2-{[(2-{[(E)-2-(dimethylamino)ethenyl](ethyl)amino}-2-oxoethyl)amino]methyl}pyridine-4-carboxylic acid | C15 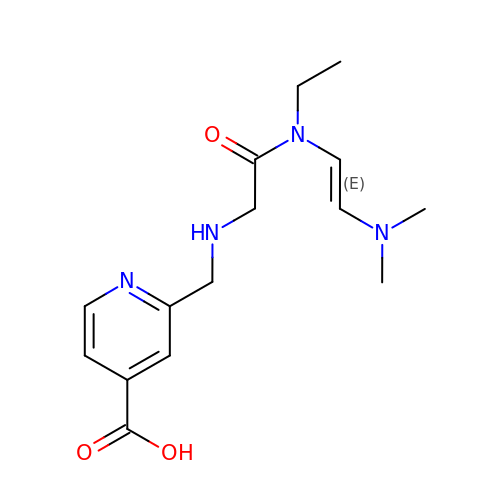H22 N4 O3 | RTKGUAPXWDCFNW-BQYQJAHWSA-N>[2x]GSMSESADLTELYSIIEKTAQVVDVTASHDKVWPILNAFQDVIADSVISFRASTGSSADDLDCRFTMLPKGLDPYARALEHGLTPKTDHPVGSLLKEVHENLPITSCGVDFGVAGGFTKTWSFPSAEKLGKVSELVKLPSIPDAVAANRDFFEKWGIADMVSTVGIDYSKRTMNLYFGGGVGDRVPAGVFEEKGVRAILGELGLAAPSEELLKFCERSFVIYVTLSWDSPKINRFTYSVMTPE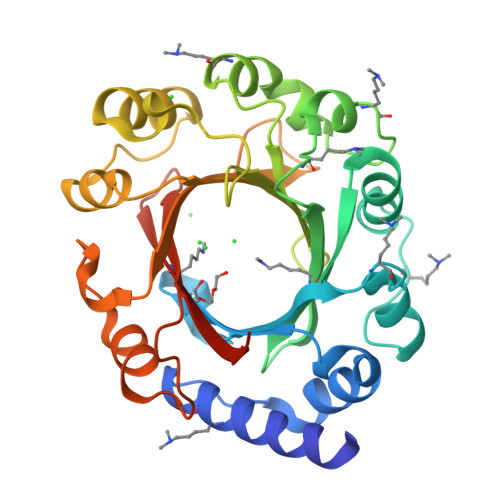PLGLPVDLAPTFERLIKSAPYDTEGRNYVYGIASTPKGEYHKIASYYQWQKRVEKLLRSDG>[2x]MAATTVNGGTVHFKGEVVNAACAVDAGSVDQTVQLGQVRTASLAQEGATSSAVGFNIQLNDCDTNVASKAAVAFLGTAIDAGHTNVLALQSSAAGSATNVGVQILDRTGAALTLDGATFSSETTLNNGTNTIPFQARYFATGAATPGAANADATFKVQYQ;> MGVALGATRVIYPAGQKQEQLAVTNNDENSTYLIQSWVENADGVKDGRFIVTPPLFAMKGKKENTLRILDATNNQLPQDRESLFWMNVKAIPSMDKSKLTENTLQLAIISRIKLYYRPAKLALPPDQAAEKLRFRRSANSLTLINPTPYYLTVTELNAGTRVLENALVPPMGESTVKLPSDAGSNITYRTINDYGALTPKMTGVME;> DLYFNPRFLADDPQAVADLSRFENGQELPPGTYRVDIYLNNGYMATRDVTFNTGDSEQGIVPCLTRAQLASMGLNTASVAGMNLLADDACVPLTTMVQDATAHLDVGQQRLNLTIPQAFMSNRARGYIPPELWDPGINAGLLNYNFSGNSVQNRIGGNSHYAYLNLQSGLNIGAWRLRDNTTWSYNSSDRSSGSKNKWQHINTWLERDIIPLRSRLTLGDGYTQGDIFDGINFRGAQLASDDNMLPDSQRGFAPVIHGIARGTAQVTIKQNGYDIYNSTVPPGPFTINDIYAAG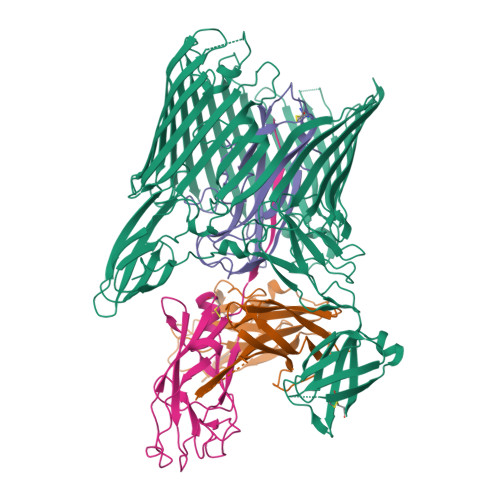NSGDLQVTIKEADGSTQIFTVPYSSVPLLQREGHTRYSITAGEYRSGNAQQEKPRFFQSTLLHGLPAGWTIYGGTQLADRYRAFNFGIGKNMGALGALSVDMTQANSTLPDDSQHDGQSVRFLYNKSLNESGTNIQLVGYRYSTSGYFNFADTTYSRMNGYNIETQDGVIQVKPKFTDYYNLAYNKRGKLQLTVTQQLGRTSTLYLSGSHQTYWGTSNVDEQFQAGLNTAFEDINWTLSYSLTKNAWQKGRDQMLALNVNIPFSHWLRSDSKSQWRHASASYSMSHDLNGRMTNLAGVYGTLLEDNNLSYSVQTGYAGGGDGNSGSTGYATLNYRGGYGNANIGYSHSDDIKQLYYGVSGGVLAHANGVTLGQPLNDTVVLVKAPGAKDAKVENQTGVRTDWRGYAVLPYATEYRENRVALDTNTLADNVDLDNAVANVVPTRGAIVRAEFKARVGIKLLMTLTHNNKPLPFGAMVTSESSQSSGIVADNGQVYLSGMPLAGKVQVKWGEEENAHCVANYQLPPESQQQLLTQLSAECRLVPRGSWSHPQFEK>[2x]MHIERLAVDESVGRAMPPQRFIEALSDLGVPVEFAGEDEQFGPGDAVASFGHRDAFLDADWVHCIRAGYDEFPVGVYEEAGTYLTNSTGIHGTTVGETVAGYMLTFARRLHAYRDAQHDHAWDLPRYEEPFTLAGERVCVVGLGTLGRGVVDRAAALGMEVVGVRRSGDPVDNVSTVYTPDRLHEAIADARFVVLATPLTDETEGMVAAPEFETMREDASLVNVARGPVVVESDLVAALDS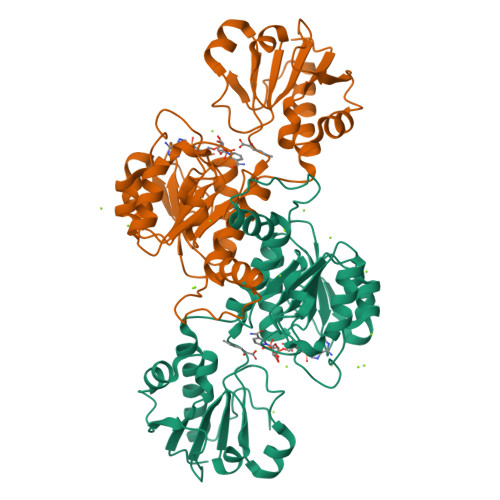GDIAGAALDVFSEEPLPEDSPLWDFEDVLITPHVSAATSKYHEDVAALIRENIEKIATGDELTNRVV> MAKLLQRVEITLRSFYIFNSTFGQVEGEEHKKVLFYHPNDIELNTKIKDVGLSEAIIRFTGTFTSEDDCQALHTQKTTQLFYQPEPGYWLVLVLNVPKEVRLKEGVEVADYRGAEISDRIYRAILRQCYQMFRFQNGCFSSCGSEEPNPDKRRELLCQKLLQFYDQHLTNLRDPAQCDIIDMLHSIQYLPLDKTLFLRAQNFGTLCETFPDIKESIMLYQEQVLCGGKLSPEDLHCVHSYVVQHVLKVEASSSTIAVSPSLKRSISECQVGGFVRSRQKVAGDEHDAVNEEDHPMKVYVTLDKEAKPYYLLIYRALHITLCLFLNADQVAPKQDLYDDLHAYMAPQLTSLARDISSELTKEAVGAAGQDNSSGNSETAPKYLFINEQSLQHHTNFQRHLPQGLPRNVLSIIADLANGSGKAEMESAPAEEVQVKTTNDYWIVKRRCNYR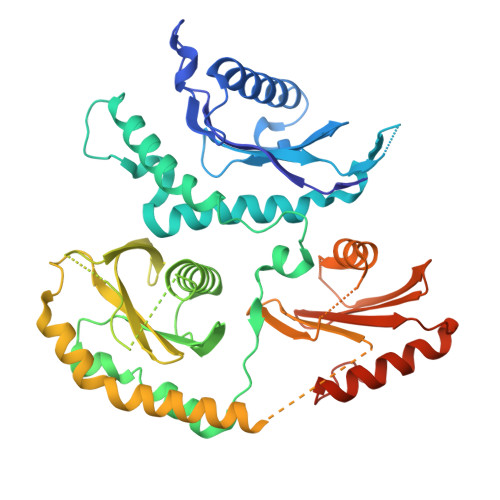QYYVILCNSKATLLDVTQEARRIFEQELTDDVFFDKDYKDHDGDYKDHDIDYKDDDDK>[2x]MPYRNCWSKIMKKLINDVQQVLDEQLAGLAKAHPSLTLHQDPVYVTRADAPVAGKVALLSGGGSGHEPMHCGYIGQGMLSGACPGEIFTSPTPDKIFECAMQVDGGEGVLLIIKNYTGDILNFETATELLHDSGVKVTTVVIDDDVAVKDSLYTAGRRGVANTVLIEKLVGAAAERGDSLDACAELGRKLNNQGHS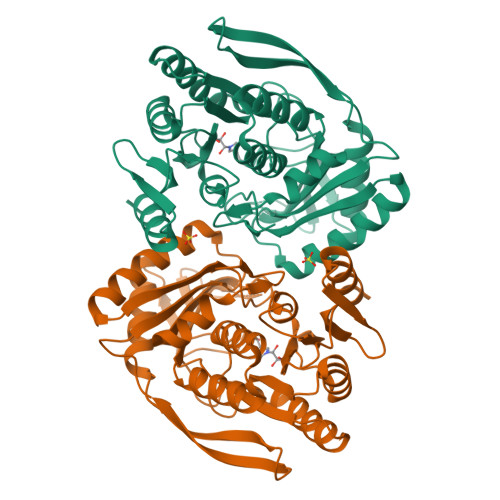IGIALGACTVPAAGKPSFTLADNEMEFGVGIHGEPGIDRRPFSSLDNTVDEMFDTLLVNGSYHRTLRFWDYQQGSWQEEQQTKQPLQSGDRVIALVNNLGATPLSELYGVYNRLTTRCQQAGLTIERNLIGAYCTSLDMTGFSITLLKVDDETLALWDAPVHTPALNWGK> MVTGMFSLGRTYLFRVPEGEELLTYIKNFCKKEGIETAIINGIGTLKNPKIGYFLEEKKEYKVIPLKGSY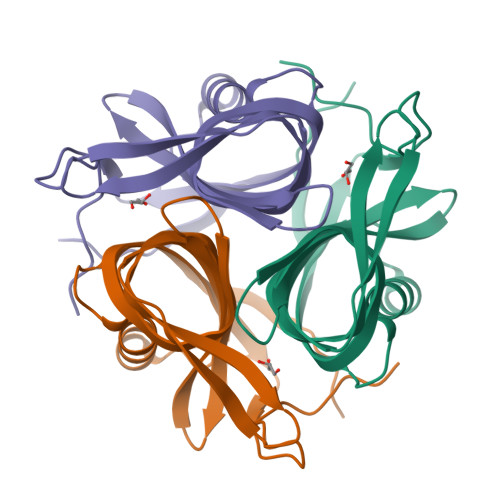ELISLIGNVSLKDGEPFVHAHVSLGNEEGIVFGGHLVEGEVFVAEIFLQELKGEKIERKPTKYGLALWEELKL> MTSLIDLGRYVERTHHGEDTEPRSKRVKIAKPDLSSFQPGSIIKIRLQDFVTYTLTEFNLSPSLNMIIGPNGSGKSTFVCAVCLGLAGKPEYIGRSKKVEDFIKNGQDVSKIEITLKNSPNVTDIEYIDARDETIKITRIITRSKRRSDYLINDYQVSESVVKTLVAQLNIQLDNLCQFLSQERVEEFARLKSVKLLVETIRSIDASLLDVLDELRELQGNEQSLQKDLDFKKAKIVHLRQESDKLRKSVESLRDFQNKKGEIELHSQLLPYVKVKDHKEKLNIYKEEYERAKANLRAILKDKKPFANTKKTLENQVEELTEKCSLKTDEFLKAKEKINEIFEKLNTIRDEVIKKKNQNEYYRGRTKKLQATIISTKEDFLRSQEILAQTHLPEKSVFEDIDIKRKEIINKEGEIRDLISEIDAKANAINHEMRSIQRQAESKTKSLTTTDKIGILNQDQDLKEVRDAVLMVREHPEMKDKILEPPIMTVSAINAQFAAYLAQCVDYNTSKALTVVDSDSYKLFANPILDKFKVNLRELSSADTTPPVPAETVRDLGFEGYLSDFITGDKRVMKMLCQTSKIHTIPVSRRELTPAQIKKLITPRPNGKILFKRIIHGNRLVDIKQSAYGSKQVFPTDVSIKQTNFYQGSIMSNEQKI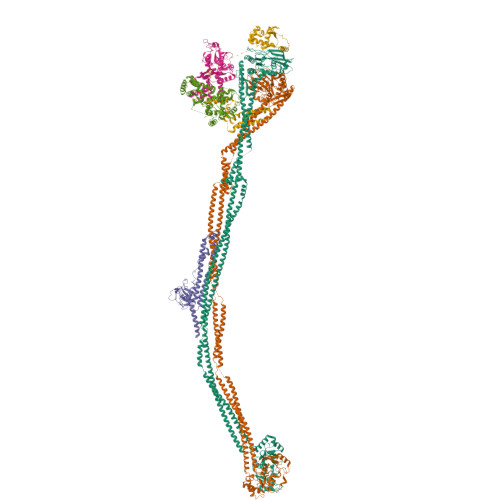RIENEIINLKNEYNDRKSTLDALSNQKSGYRHELSELASKNDDINREAHQLNEIRKKYTMRKSTIETLREKLDQLKREARKDVSQKIKDIDDQIQQLLLKQRHLLSKMASSMKSLKNCQKELISTQILQFEAQNMDVSMNDVIGFFNEREADLKSQYEDKKKFVKEMRDTPEFQSWMREIRSYDQDTKEKLNKVAEKYEEEGNFNLSFVQDVLDKLESEIAMVNHDESAVTILDQVTAELRELEHTVPQQSKDLETIKAKLKEDHAVLEPKLDDIVSKISARFARLFNNVGSAGAVRLEKPKDYAEWKIEIMVKFRDNAPLKKLDSHTQSGGERAVSTVLYMIALQEFTSAPFRVVDQINQGMDSRNERIVHKAMVENACAENTSQYFLITPKLLTGLHYHEKMRIHCVMAGSWIPNPSEDPKMIHFGETSNYSFD;> MISTTISGKRPIEQVDDELLSLTAQQENEEQQQQRKRRRHQFAPMTQFNSNTLDEDSGFRSSSDVATADQDNFLEESPSGYIKKVILRNFMCHEHFELELGSRLNFIVGNNGSGKSAILTAITIGLGAKASETNRGSSLKDLIREGCYSAKIILHLDNSKYGAYQQGIFGNEIIVERIIKRDGPASFSLRSENGKEISNKKKDIQTVVDYFSVPVSNPMCFLSQDAARSFLTASTSQDKYSHFMKGTLLQEITENLLYASAIHDSAQENMALHLENLKSLKAEYEDAKKLLRELNQTSDLNERKMLLQAKSLWIDVAHNTDACKNLENEISGIQQKVDEVTEKIRNRQEKIERYTSDGTTIEAQIDAKVIYVNEKDSEHQNARELLRDVKSRFEKEKSNQAEAQSNIDQGRKKVDALNKTIAHLEEELTKEMGGDKDQMRQELEQLEKANEKLREVNNSLVVSLQDVKNEERDIQHERESELRTISRSIQNKKVELQNIAKGNDTFLMNFDRNMDRLLRTIEQRKNEFETPAIGPLGSLVTIRKGFEKWTRSIQRAISSSLNAFVVSNPKDNRLFRDIMRSCGIRSNIPIVTYCLSQFDYSKGRAHGNYPTIVDALEFSKPEIECLFVDLSRIERIVLIEDKNEARNFLQRNPVNVNMALSLRDRRSGFQLSGGYRLDTVTYQDKIRLKVNSSSDNGTQYLKDLIEQETKELQNIRDRYEEKLSEVRSRLKEIDGRLKSTKNEMRKTNFRMTELKMNVGKVVDTGILNSKINERKNQEQAIASYEAAKEELGLKIEQIAQEAQPIKEQYDSTKLALVEAQDELQQLKEDINSRQSKIQKYKDDTIYYEDKKKVYLENIKKIEVNVAALKEGIQRQIQNACAFCSKERIENVDLPDTQEEIKRELDKVSRMIQKAEKSLGLSQEEVIALFEKCRNKYKEGQKKYMEIDEALNRLHNSLKARDQNYKNAEKGTCFDADMDFRASLKVRKFSGNLSFIKDTKSLEIYILTTNDEKARNVDTLSGGEKSFSQMALLLATWKPMRSRIIALDQFDVFMDQVNRKIGTTLIVKKLKDIARTQTIIITPQDIGKIADIDSSGVSIHRMRDPERQNNSNFYN;> MGSYPYDVPDYAGSGALNDNPIPKSVPLHPKSGKYFHNLHARDLSNIYQQCYKQIDETINQLVDSTSPSTIGIEEQVADITSTYKLLSTYESESNSFDEHIKDLKKNFKQSSDACPQIDLSTWDKYRTGELTAPKLSELYLNMPTPEPATMVNNTDTLKILKVLPYIWNDPTCVIPDLQNPADEDDLQIEGGKIELTCPITCKPYEAPLISRKCNHVFDRDGIQNYLQGYTTRDCPQAACSQVVSMRDFVRDPIMELRCKIAKMKESQEQDKRSSQAIDVL;> MGSSHHHHHHSSGRENLYFQGHMEVHEEQVSAPVTGDATAKYLLQYILSARGICHENALILALMRLETDASTLNTEWSIQQWVDKLNDYINAINVKLNLLGYKIIRINHGIGRNAVTLKAKQNFESFEDNTAIRAHNNDYAVLQSIVLPESNRFFVYVNLASTEETKLATRFNQNEIEFMKWAIEQFMISGETIVEGPALETSIIVKEVNRILVAATGDSNLAKWRKFSTFTVGSTNLFQFQELTATDIEDLLLRLCELKWFYRTQEGKFGIDLRCIAELEEYLTSMYNLNTCQNCHKLAIQGVRCGNESCREENEETGENSLSQIWHVDCFKHYITHVSKNCDRCGSSLITEGVYVI;> MSSIDNDSDVDLTEDLAVAKIVKENPVARKMVRYILSRGESQNSIITRNKLQSVIHEAAREENIAKPSFSKMFMDINAILYNVYGFELQGLPSKNNMNAGGNGSNSNTNKSMPEPLGHRAQKFILLNNVPHSKNFDDFKILQSAHTYEELIVTGEYIGDDIASGTSNTLESKLSTDRDLVYKGVLSVILCIVFFSKNNILHQELIKFLETFGIPSDGSKIAILNITIEDLIKSLEKREYIVRLEEKSDTDGEVISYRIGRRTQAELGLESLEKLVQEIMGLEKEQTKSLHDDIIKSIGDSYSI;> MSSTVISRKRRNSTVTEPDSSGETRKQKKSRSDEKSSSSKDGDPQLEFKVLQGYRDLESEMHKGRAQVTRTGDIGVAMDNLNAVDSLFNKVIGIKNNGLFAHDARAMVSISELAQISVRNLKFDDSRSMVNLENIVNSLKRYMLKEHFKLNNIAENRNDLTLAADEQSAADQQEESDGDIDRTPDDNHTDKATSSFKATSMRHSYLQQFSHYNEFSQFNWFRIGALYNTISKNAPITDHLMGPLSIEKKPRVLTQRRRNNDQVGEKITAEKITQHSLNSTQQETTPEQVKKCFKKLSKKLGPEGSINLFKFIIDPNSFSRSIENLFYTSFLIKEGKLLMEHDEEGLPTIKIKQSISHTDSRSKEIERQRRRAAHQNHIIFQMDMPTWRKLIKKYNITSPFLDGSSGMAEIGTGFPFDPHYVEVLGERMHYVDVGPRDGTPVLFLHGNPTSSYVWRNIIPHVAPTHRCIAPDLIGMGKSDKPDLGYFFDDHVRFMDAFIEALGLEEVVLVIHDWGSALGFHWAKRNPERVKGIAFMEFIRPIPTWDEWPEFARETFQAFRTTDVGRKLIIDQNVFIEGTLPMGVVRPLTEVEMDHYREPFLNPVDREPLWRFPNELPIAGEPANIVALVEEYMDWLHQSPVPKLLFWGTPGVLIPPAEAARLAKSLPNCKAVDIGPGLNLLQEDNPDLIGSEIARWLSTLEISGGSEQKLISEEDL> MSQAATPAADGKVKISIDPLTRVEGHLKIEVEVKDGKVVDAKCSGGMFRGFEQILRGRDPRDSSQIVQRICGVCPTAHCTASVMAQDDAFGVKVTTNGRITRNLIFGANYLQSHILHFYHLAALDYVKGPDVSPFVPRYANADLLTDRIKDGAKADATNTYGLNQYLKALEIR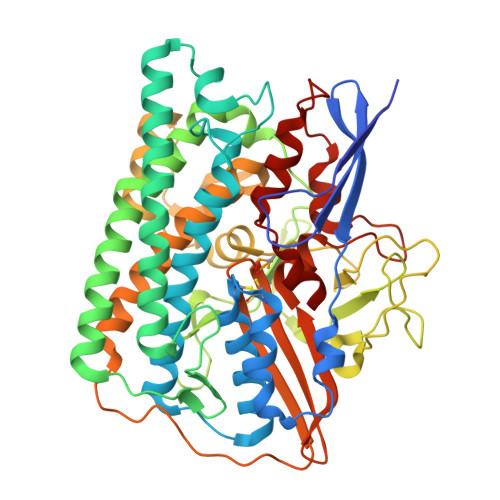RICHEMVAMFGGRMPHVQGMVVGGATEIPTADKVAEYAARFKEVQKFVIEEYLPLIYTLGSVYTDLFETGIGWKNVIAFGVFPEDDDYKTFLLKPGVYIDGKDEEFDSKLVKEYVGHSFFDHSAPGGLHYSVGETNPNPDKPGAYSFVKAPRYKDKPCEVGPLARMWVQNPELSPVGQKLLKELYGIEAKNFRDLGDKAFSIMGRHVARAEETWLTAVAVEKWLKQVQPGAETYVKSEIPDAAEGTGFTEAPRGALLHYLKIKDKKIENYQIVSATLWNANPRDDMGQRGPIEEALIGVPVPDIKNPVNVGRLVRSYDPULGCAVH Integral membrane proteins belonging to the multidrug and toxic compound extrusion (MATE) family contribute to multidrug resistance by using either the Na+ or H+ electrochemical gradient to extrude drugs across cell membranes. MATE proteins identified thus far can be separated into the NorM, DinF and eukaryotic subfamilies based on amino-acid sequence similarity. Those crystal structures revealed a similar protein fold comprising 12 membrane-spanning segments (TM1-TM12), they nevertheless suggested different arrangement of cation- and substrate-binding sites between the NorM and DinF proteins, hinting at substantial mechanistic diversity among the MATE transporters.

To reveal how verapamil blocks drug binding, we co-crystallized DinF-BH with verapamil, and determined the co-structure to 3.0 Å resolution by using molecular replacement and MIRAS phasing. The structure of verapamil-bound, extracellular-facing DinF-BH is very similar to that of the R6G-bound form9, with an r.m.s.d. of <0.5 Å for 447 Cα positions. About half-way across the membrane bilayer, verapamil adopts a rather extended conformation and makes numerous close-range interactions with both the N (TM1-TM6) and C (TM7-TM12) domains of DinF-BH. Specifically, the side chains of N37 (TM1) and Q252 (TM7) form H-bonds with the bound verapamil, whereas those of M33, Y36 (TM1), F60, M63, M64, M67 (TM2), F150, F154 (TM4), M286 and M293 (TM8) make contacts through van der Waals interactions. Moreover, although the positively charged verapamil is enclosed in a binding chamber with an overall negative surface electrostatic potential, no close-range ionic interaction could be found between DinF-BH and verapamil. Structural comparison of the verapamil- and R6G-bound DinF-BH revealed overlapping, but not identical, binding sites for both ligands. Notably, all the verapamil-contacting amino acids except M64, Q252 and M293 make contacts with R6G. Therefore, the binding of verapamil and R6G to DinF-BH is mutually exclusive, offering a structural rationale for the obstruction of multidrug efflux by verapamil. By contrast, in the verapamil-bound structure, D40 is positioned ∼9 Å away from atom N8 in verapamil, the ternary ammonium group carrying a positive charge. Therefore, verapamil may interact with D40 through long-range electrostatic forces, which is likely enabled by the hydrophobic, low dielectric environment within the membrane-embedded drug-binding chamber.

> MEQKQQSERLGTEAIPKLLRSLSIPAMIGMFVMALYNVVDTIFISYAVGIEGVAGVTIAFPIMMIMMSMAGALGIGGASVISRRLGERRGEEANQVFGNILTVILVLSVIGFISAFTLLGPALQLFGATSVTQGYATDYLFPILLGSIFFFFAFAANNIIRSEGNATFAMVTMIVPAVLNILLDVLFIFGLNMGVLGASIATVIAQASVTGLVLRYFLTGKSTLSLHWSDLRMKGSVIKEVCLVGLPAFVQQSSASLMMIAINSMLLRFGSDFYVGVFGLVQRIMMFVMMPMMGIMQAMQPIVGYNYGAKQYSRLRETVMLGFKVATIFSIGIFALLMLFPEALLRVFTADREVIQAGVSAMHILFCVTFLIGAQIVAGGLYQSLGKPKQALILSLSRQIIFLIPLVLILPHIFGLSGVWWAFPIADVLSFILTVVLLYRDRNVFFLKTKEERELDLVKTASST>[2x]MSNLKDFSQPGSGQESNFGVDFVIHYKVPAAERDEAEAGFVQLIRALTTVGLATEVRHGENESLLVFVKVASPDLFAKQVYRARLGDWLHGVRVSAPHNDIAQALQDEPVVEAERLRLIYLMITKPHNEGGAGVTPTNAKWKHVESIFPLHSHSFNKEWIKKWSSKYTLEQTDIDNIRDKFGESVAFYFAFLRSYFRFLVIPSAFGFGAWLLLGQFSYLYALLCGLWSVVFFEYWKKQEVDLAVQWGVRGVSSIQQSRPEFEWEHEAEDPITGEPVKVYPPMKRVKTQLLQIPFALACVVALGALIVTCNSLEVFINEVYSGPGKQYLGFLPTIFLVIGTPTISGVLMGAAEKLNAMENYATVDAHDAALIQKQFVLNFMTSYMALFFTAFVYIPFGHILHPFLNFWRATAQTLTFSEKELPTREFQINPARISNQMFYFTVTAQIVNFATEVVVPYIKQQAFQKAKQLKSGSKVQEDHEE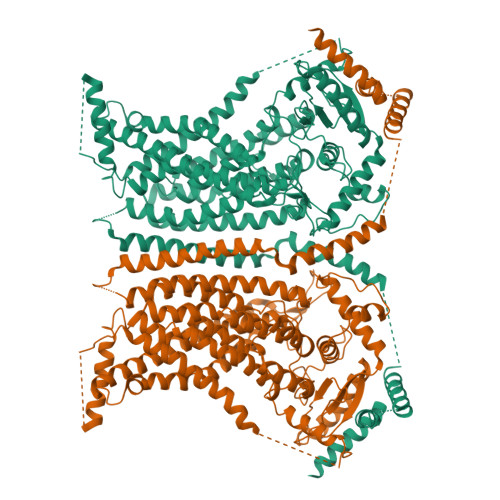EAEFLQRVREECTLEEYDVSGDYREMVMQFGYVAMFSVAWPLAACCFLVNNWVELRSDALKIAISSRRPIPWRTDSIGPWLTALSFLSWLGSITSSAIVYLCSNSKNGTQGEASPLKAWGLLLSILFAEHFYLVVQLAVRFVLSKLDSPGLQKERKERFQTKKRLLQENLGQDAAEEAAAPGIEHSEKITREALEEEARQASIRGHGTPEEMFWQRQRGMQETIEIGRRMIEQQLAAGKNGKKSAPAVPSEKAS Matrix metalloproteinase 1 (MMP-1) plays a pivotal role in degradation of interstitial collagen types I, II, and III. Under normal physiological conditions, MMP activity can be regulated at various stages: during transcription, proteolytic processing of their inactive pro forms, zymogens, as well as by inhibition of enzyme activity by endogenous inhibitors such as tissue inhibitors of metalloproteinases or TIMPs. These enzymes have a similar domain structure: an N-terminal signal sequence to target for secretion, a pro-peptide domain to maintain latency, a catalytic domain containing the catalytic zinc, a linker region, and a C-terminal four-bladed propeller structure called the hemopexin domain. The collagenases cleave the triple-helical collagen approximately three-quarters away from the N terminus of the substrate, resulting in three-quarters and one quarter length fragments that are unstable at body temperature and undergo denaturation, rendering them susceptible to other non-specific tissue proteinases. The proteolytic activity of the enzyme resides in the catalytic domain but it requires the hemopexin domain in order to cleave the three chains of the triple-helical collagen.

It must be mentioned here that the present structure is an active site mutant where the catalytic glutamate residue has been mutated to an alanine. The structure comprises of the N-terminal catalytic domain, the linker region and the C-terminal hemopexin domain. The active site zinc is bound in the sequence HELGHXXGXXH by the three His residues: His199, His203, His209 and a water molecule at the active site cleft. The present structure on the other hand stands unique in being elucidated in the absence of an inhibitor. This is the first unliganded structure of the full-length MMP-1 where a water molecule is seen at the active site providing the fourth ligand for the catalytic zinc in the tetrahedral coordination sphere. Also observed in this domain is the salt bridge between the ammonium group of the N-terminal, Phe81 and the carboxylate group of the side-chain of Asp232. The catalytic domain of MMP-1 also contains three calcium-binding sites. In essence, the hemopexin-like domain undergoes a major displacement towards the catalytic domain, thus widening the cleft between the proteinase domain and the hemopexin-like domain on the active site face of the enzyme. This altered configuration makes the active site residues and the RWTNNFREY (residues 183–191) interface, a segment critical for collagenolysis, more accessible for native collagen.

>[2x]FVLTEGNPRWEQTHLTYRIENYTPDLPRADVDHAIEKAFQLWSNVTPLTFTKVSEGQADIMISFVRGDHRDNSPFDGPGGNLAHAFQPGPGIGGDAHFDEDERWTNNFREYNLHRVAAHALGHSLGLSHSTDIGALMYPSYTFSGDVQLAQDDIDGIQAIYGRSQNPVQPIGPQTPKACDSKLTFDAITTIRGEVMFFKDRFYMRTNPFYPEVELNFISVFWPQLPNGLEAAYEFADRDEVRFFKGNKYWAVQGQNVLHGYPKDIYSSFGFPRTVKHIDAALSEENTGKTYFFVANKYWRYDEYKRSMDPGYPKMIAHDFPGIGHKVDAVFMKDGFFYFFHGTRQYKFDPKTKRILTLQKANSWFNC> MMRRMWVPTFSAQQQHLHHAMVLKMSTYASTPSGNGVTSAASNEEMNLHDAAAIAPGPYRRVGNIFIVHCDDHPFKHSWEVNRMLRELRLEFKGQTTIVPDIPQVRKRIWRVRHIVKVDVLDLDEAKALIGVPEHISFTDLASQLPPSFGRVKAVPSPVIRSKMNFMKLRRMRLRDVLHRDALELRLLELKRSAMKN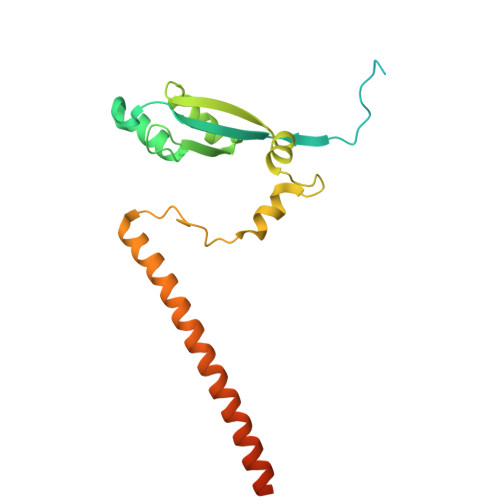AEQQKHAQKDERTDNKEGEKC The bacterial periplasmic methionine‐binding protein MetQ is involved in the import of methionine by the cognate MetNI methionine ATP binding cassette (ABC) transporter. MetQ, the substrate‐binding protein (SBP) for MetNI,5, 6 is proposed to play a dual role in transport by either binding l‐methionine for delivery to the translocation pathway of MetNI, or by facilitating d‐methionine uptake through the ligand‐free form when complexed to the transporter. Structural studies of SBPs in their ligand‐bound and ligand‐free forms have revealed a hinge‐bending or “Venus‐flytrap” mechanism where two domains of SBPs adopt their open conformation with an accessible binding site in the absence of substrate; substrate binding stabilizes the closed conformation, where the two domains come together and sequester the substrate. In this study, we report the structures of the Neisseria meningitides MetQ in substrate‐free form and in complexes with l‐methionine and with d‐methionine, along with the associated binding constants determined by isothermal titration calorimetry.

With the exception of MetQ found in the MetNIQ complex, the structure of substrate‐free MetQ has not been reported. Since MetQ has a high affinity for l‐methionine, preparation of the apo‐MetQ requires cycles of unfolding and refolding to remove the bound ligand. As an alternative approach, mutation of Asn229 to Ala (N229A) in the binding pocket of the E. coli MetQ was found to substantially decrease the affinity toward methionine, thereby greatly facilitating preparation of the substrate‐free form of MetQ. Despite extensive efforts with both approaches, we could not crystallize the substrate‐free form of E. coli MetQ. Structures of the substrate‐free (N238A) and substrate‐bound N. meningitides MetQ are related by a “Venus‐fly trap” hinge‐type movement of the two domains accompanying methionine binding and dissociation. l‐ and d‐methionine bind to the same site on MetQ, and this study emphasizes the important role of asparagine 238 in ligand binding and affinity. As this asparagine residue interacts with both the α‐amino and α‐carboxyl groups of l‐methionine, mutation to alanine would be expected to significantly impair ligand binding. Three distinct conformational states have been characterized to date for MetQ: one liganded and two ligand‐free forms. A thermodynamic analysis demonstrates that ligand‐free MetQ associates with the ATP‐bound form of MetNI ∼40 times more tightly than does liganded MetQ, consistent with the necessity of dissociating methionine from MetQ for transport to occur.

> EIVFGTTVGDFGDMVKEQIQAELEKKGYTVKLVEFTDYVRPNLALAEGELDINVFQHKPYLDDFKKEHNLDITEVFQVPTAPLGLYPGKLKSLEEVKDGSTVSAPNDPSNFARVLVMLDELGWIKLKDGINPLTASKADIAENLKNIKIVELEAAQLPRSRADVDFAVVNGNYAISSGMKLTEALFQEPSFAYVAWSAVKTADKDSQWLKDVTEAYNSDAFKAYAHKRFEGYKSPAAWNEG> MPQYQTWEEFSRAAEKLYLADPMKA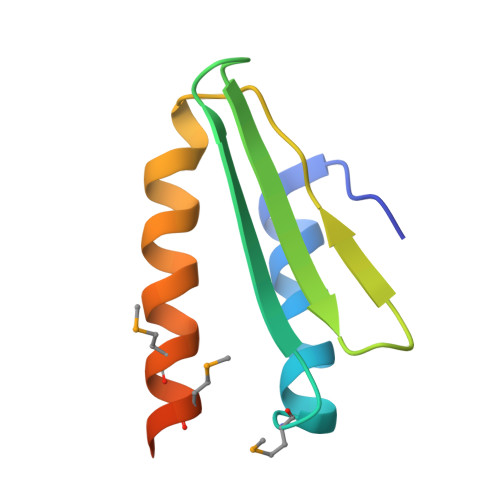RVVLKYRHSDGNLCVKVTDDLVCLVYKTDQAQDVKKIEKFHSQLMRLMVAKEARNVTMET>[2x]MVAAPPAVGAAMPSLDFDTSVFNKEKVSLAGHEEYIVRGGRNLFPLLPEAFKGIKQIGVIGWGSQGPAQAQNLRDSLAEAKSDIVVKIGLRKGSKSFDEARAAGFTEESGTLGDIWETVSGSDLVLLLISDAAQADNYEKIFSHMKPNSILGLSHGFLLGHLQSAGLDFPKNISVIAVCPKGMGPSVRRLYVQGKEINGAGINSSFAVHQDVDGRATDVALGWSVALGSPFTFATTLEQEYKSDIFGERGILLGAVHGIVEALFRRYTEQGMDEEMAYKNTVEGITGIISKTISKKGMLEVYNSLTEEGKKEFNKAYSASFYPCMDILYECYEDVASGSEIRSVVLAGRRFYEKEGLPAFPMGNIDQTRMWKVGEKVRSTRPENDLGPLHPFTAGVYVALMMAQIEVLRKKGHSYSEIINESVIESVDSLNPFMHARGVA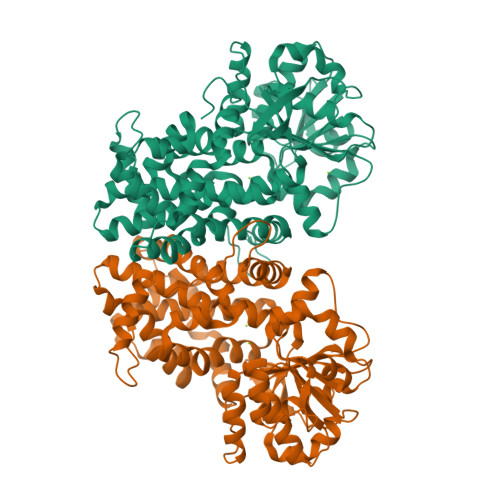FMVDNCSTTARLGSRKWAPRFDYILTQQAFVTVDKDAPINQDLISNFMSDPVHGAIEVCAELRPTVDISVPANADFVRPELRQSS>VA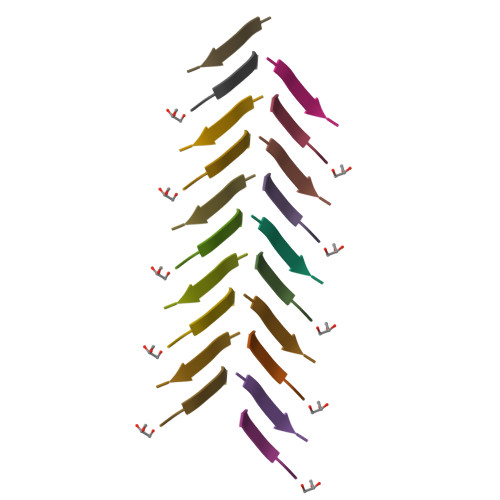VHVF[2x]>[2x]MSEFSQTVPELVAWARKNDFSISLPVDRLSFLLAVATLNGERLDGEMSEGELVDAFRHVSDAFEQTSETIGVRANNAINDMVRQRLLNRFTSEQAEGNAIYRLTPLGIGITDYYIRQREFSTLRLSMQLSIVAGELKRAADAAEEGGDEFHWHRNVYAPLKYSVAEIFDSIDLTQRLMDEQQQQVKDDIAQLLNKDWRAAISSCELLLSETSGTLRELQDTLEAAGDKLQANLLRIQDATMTHDDLHFVDRLVFDLQSKLDRIISWGQQSIDLWIGYDRHVHKFIRTAIDMDKNRVFAQRLRQSVQTYFDEPWALTYANADRLLDMRDEEMALRDEEVTGELPEDLEYEEFNEIREQLAAIIEEQLAVYKTRQVPLDLGLVVREYLSQYPRARHFDVARIVIDQAVRLGVAQADFTGLPAKWQPINDYGAKVQAHVIDKY;>[2x]MSSTNIEQVMPVKLAQALANPLFPALDSALRSGRHIGLDELDNHAFLMDFQEYLEEFYARYNVELIRAPEGFFYLRPRSTTLIPRSVLSELDMMVGKILCYLYLSPERLANEGIFTQQELYDELLTLADEAKLLKLVNNRSTGSDVDRQKLQEKVRSSLNRLRRLGMVWFMGHDSSKFRITESVFRFGADVRAGDDPREAQRRLIRDGEAMPIENHLQLNDETEENQPDSGEEE;>GPGMSRDLVTIPRDVWNDIQGYIDSLERENDSLKNQLMEADEYVAELEEKLNGTS[2x]

MukBEF folds the chromosome of Escherichia coli and related bacteria. The SMC protein MukB dimerizes at its ‘‘hinge’’ domain, which connects via the long coiled-coil ‘‘arm’’ to the ABC-type ATPase ‘‘head’’ domain. The heads are bridged by the kleisin MukF, whereby the C-terminal winged-helix domain (cWHD) of MukF binds the ‘‘cap’’ surface of one MukB, and the N-terminal middle domain (MD) binds the coiled-coil ‘‘neck’’ of the other MukB. MukF also recruits the dimeric KITE protein MukE.

Focused classification, signal subtraction of the MukF core, and focused refinement using neural-network-based regularization with Blush resolved a 73 kDa region of MukE bound to gp5.9. As observed previously in its RecBCD-bound form, gp5.9 formed a parallel coiled-coil dimer complemented by a β sheet of the N-terminal strands. gp5.9 bound along the DNA-binding cleft of MukE, overlapping along its full length with the DNA capture site. However, the orientation of gp5.9 with respect to the DNA molecule is broadly similar, in the sense that the long axis of the gp5.9 coiled coil aligns approximately with that of the double helix. Moreover, within the resolution limits of the structures, gp5.9 positioned several negatively charged residues (D11, D15, D21, E24, E36, D38, E43, and E45) near positively charged residues in MukE (R140, K150, R163, R164, and R179) or MukF (R322). Most of these ion pair interactions mimic DNA phosphate backbone contacts and thus prevent the natural DNA substrate from binding efficiently. Therefore, although there are significant differences in the details of binding to individual targets, the data overall support the designation of gp5.9 as a DNA mimic protein. The structure revealed that binding of gp5.9 to the MukE DNA-binding cleft is mutually exclusive with formation of the DNA capture state. We find that gp5.9 targets the DNA-binding site of MukE, which contacts DNA both in the capture state and when DNA is entrapped in the clamp compartment. Although gp5.9 targets DNA-binding sites by contacting residues involved in phosphate backbone binding, it encodes sufficient specificity to interfere with select targets.> NAINPRLTPWTYRNTSFSSLPLTGENPGAWALVRDNSAKGITAGSGSQQTTYDPTRTEAALTASTTFALRRYDLAGRALYDLDFSKLNPQTPTRDQTGQITFNPFGGFGLSGAAPQQWNEVKNKVPVEVAQDPSNPYRFAVLLVPRSVVYYEQLQRGLGLPQQRTESGQNTSTTGAMFGLKVKNAEADTAKSNEKLQGAEATGSSTTSGSGQSTQRGGSSGDTKVKALKIEVKKKSDSEDNGQLQLEKNDLANAPIKRSEESGQSVQLKADDFGTALSSSGSGGNSNPGSPTPWRPWLATEQIHKDLPKWSASILILYDAPYARNRTAIDRVDHLDPKAMTANYPPSWRTPKWNHHGLWDWKARDVLLQTTGFFNPRRHPEWFDGGQTVADNEKTGFDVDNSENTKQGFQKEADSDKSAPIALPFEAYFANIGNLTWFGQALLVFGGNGHVTKSAHTAPLSIGVFRVRYNATGTSATVTGWPYALLFSGMVNKQTDGLKDLPFNNNRWFEYVPRMAVAGAKFVGRELVLAGTITMGDTATVPRLLYDELESNLNLVAQGQGLLREDLQLFTPYGWANRPDLPIGAWSSSSSSSHNAPYYFHNNPDWQDRPIQNVVDAFIKPWEDKNGKDDAKYIYPYRYSGMWAWQVYNWSNKLTDQPLSADFVNENAYQPNSLFAAILNPELLAALPDKVKYGKENEFAANEYERFNQKLTVAPTQGTNWSHFSPTLSRFSTGFNLVGSVLDQVLDYVPWIGNGYRYGNNHRGVDDITAPQTSAGSSSGISTNTSGSRSFLPTFSNIGVGLKANVQATLGGSQTMITGGSPRRTLDQANLQLWTGAGWRNDKASSGQSDENHTKFTSATGMDQQGQSGTSAGNPDSLKQDNISKSGDSLTTQDGNAIDQQEATNYTNLPPNLTPTADWPNALSFTNKNNAQRAQLFLRGLLGSIPVLVNRSGSDSNKFQATDQKWSYTDLHSDQTKLNLPAYGEVNGLLNPALVETYFGNTRAGGSGSNTTSSPGIGFKIPEQNNDSKATLITPGLAWTPQDVGNLVVSGTTVSFQLGGWLVTFTDFVKPRAGYLGLQLTGLDASDATQRALIWAPRPWAAFRGSWVNRLGRVESVWDLKGVWADQAQSDSQGSTTTATRNALPEHPNALAFQVSVVEASAYKPNTSSGQTQSTNSSPYLHLVKPKKVTQSDKLDDDLKNLLDPNQVRTKLRQSFGTDHSTQPQPQSLKTTTPVFGTSSGNLSSVLSGGGAGGGSSGSGQSGVDLSPVEKVSGWLVGQLPSTSDGNTSSTNNLAPNTNTGNDVVGVGRLSESNAAKMNDDVDGIVRTPLAELLDGEGQTADTGPQSVKFKSPDQIDFNRLFTHPVTDLFDPVTMLVYDQYIPLFIDIPASVNPKMVRLKVLSFDTNEQSLGLRLEFFKPDQDTQPNNNVQVNPNNGDFLPLLTASSQGPQTLFSPFNQWPDKHHHHHH

M. pneumoniae binds to host target cells by means of a polar structure known as the attachment organelle, and glides in the direction of this differentiated structure at a speed of ~1 µm/s. P1, together with the P40/P90 polypeptides, forms a transmembrane complex called the “Nap”. In the present work, we report the structures of M. pneumoniae proteins P1 and P40/P90 and of complexes of P40/P90 bound to sialylated oligosaccharides. The structural results reveal that P1 (1627 residues) and P40/P90 (1218 residues) present a similar overall organization and topology in the extracellular regions.

Crystals were obtained of the M. pneumoniae Nap protein P1 extracellular region (residues Thr29-Asp1521). This P1 construct, empirically chosen after many crystallization attempts, excludes the predicted N-end of the signal secretion peptide (spanning residue Met1 to Leu59 according to the structural properties prediction program Psipred26). In this construct are also excluded the (predicted) transmembrane and intracellular regions at the C-end of P1 (residues Tyr1522 to Ala1627). The structure of P1 consists of a large N-terminal domain, with Asn60 as the first residue visible in the X-ray and the cryo-EM maps, and a smaller C-terminal domain (residues Gly1395–Asp1521). The N-terminal domain of P1 has a β-sheet propeller topology of seven consecutive blades or β-sheets, each with four antiparallel strands, except for β-sheet VII that contains only two strands. The longest intra and inter β-sheet connections cluster together creating a crown-like structure on one side of the β-propeller opposite to the position where the C-terminal domain is located. In the crown there are 13 disordered loops, spanning 117 residues, which could not be built. The C-terminal domain contains only one disordered loop (residues Thr1483–Asn1495) and has an elongated fold with the same unique topology (according to DALI29) as the C-terminal domain of adhesin P110 from M. genitalium. In the crystal structure, the C-terminal domain is anchored by crystal contacts and the density is clear and crisp, while in the top part of the crown, with few crystal contacts, temperature factors are high and chain tracing was difficult.> MSHHHHHHSMMSDLQGRKIFKVFNQDFIVDERYTVTKELGQGAYGIVCAAVNNQTSEGVAIKKVTNVFSKKILAKRALREIKLLQHFRGHRNITCLYDMDIPRPDNFNETYLYEELMECDLAAIIRSGQPLTDAHFQSFIYQILCGLKYIHSANVLHRDLKPGNLLVNADCELKICDFGLARGFSVDPEENAGYMTEYVATRWYRAPEIMLSFQSYTKAIDVWSVGCILAELLGGRPFFKGRDYVDQLNQILHILGTPNEETLSRIGSPRAQEYVRNLPFMAKKPFPTLFPNANPDALDLLDRMLAFDPSSRISVEQALEHPYLH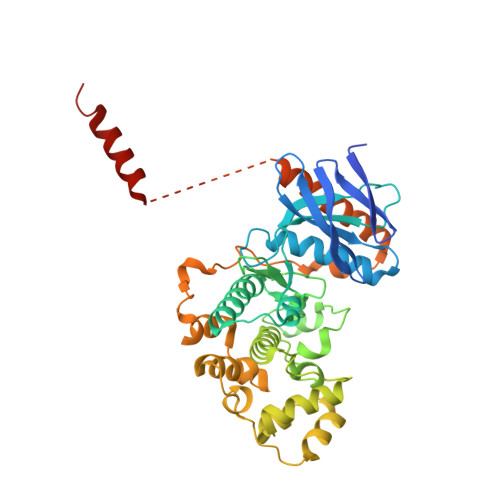IWHDASDEPDCPTTFNFDFEVVEDVGEMRKMILDEVYRFRQLVRTAPGAGGHGAPHAPQVPIPAGAGQGQWKAEDPRPQEYVGQMNDLEAELAGGLDQRR>MGQIVTFFQEVPHVIEEVMNIVLIALSVLAVLKGLYNFATCGLVGLVTFLLLCGRSCT[3x];>[3x]GTFTWTLSDSEGKDTPGGYCLTRWMLIEAELKCFGNTAVAKCNEKHDEEFCDMLRLFDFNKQAIQRLKAEAQMSIQLINKAVNALINDQLIMKNHLRDIMGIPYCNYSKYWYLNHTTTGRTSLPKCWLVSNGSYLNETHFSDDIEQQADNMITEMLQKEYMERQGKTPLGLVDLFVFSTSFYLISIFLHLVKIPTHRHIVGKSCPKPHRLNHMGICS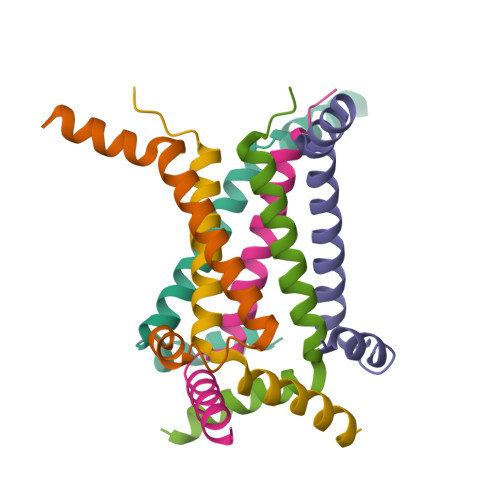CGLYKQPGVPVKWKR> MAMKREQTIENLYQLAQLTQQVQADRIEIVLEERRDEHFPPMSKALMETRSGLTRRKLDEAIAKMEEAGHQFTKNNANHYSISLSEAHMLMDAAGVPKFHERKKNNENKPWIINVQNQKGGTGKSMTAVHLAACLALNLDKRYRICLIDLDPQGSLRLFLNPQISLAEHTNIYSAVDIMLDNVPDGVQVDTEFLRKNVMLPTQYPNLKTISAFPEDAMFNAEAWQYLSQNQSLDIVRLLKEKLIDKIASDFDIIMIDTGPHVDPLVWNAMYASNALLIPCAAKRLDWASTVNFFQHLPTVYEMFPEDWKGLEFVRLMPTMFEDDNKKQVSVLTEMNYLLGDQVMMATIPRSRAFETCADTYSTVFDLTVNDFEGGKKTLATAQDAVQKSALELERVLHSHWSSLNQG

Bacterial cells use several evolutionarily-distinct genome segregation systems, the most common of which is the type I Par system. It consists of an adapter protein, ParB, that binds to the DNA cargo via interaction with the parS DNA sequence; and an ATPase, ParA, that binds nonspecific DNA and mediates cargo transport. Each chromosome encodes its own segregation complex, with Chr1 encoding a chromosomal type Ib system, and Chr2 encoding a plasmid-like type Ia system. In this study, we have reported the structure of the ParA2vc protein, in three states: apo, nucleotide-bound (ADP) and in a filamentous complex with nucleotide and DNA.

The purified protein crystallized readily, and the obtained crystals diffracted to ~2.5 Å. The obtained ParA2vc crystal structure includes one ParA2vc molecule per asymmetric unit. The overall structure of the ParA2vc monomer is similar to that of P7 ParA, with an overall RMSD of 2.2 Å for CA atoms. In particular, the N-terminal HTH domain resembles that of P1 and P7 ParA, confirming that ParA2vc belongs to the type Ia family. No ligand density was observed in the active site, confirming that this structure corresponds to the apo state of the protein. It is worth noting that the nucleotide-binding site is generally poorly resolved, and in particular we were not able to build the P-loop in this structure. One of the symmetry-related pairs is consistent with a biological dimer, and largely resembles the P7 ParA dimer structure. This suggests that we have obtained the structure of the ParA2vc dimer through crystallographic symmetry. Comparing the ParA2vc dimer to that of the P7 ParA structure confirms that they possess a similar architecture, with helix 1 forming a domain-swapped interaction with the adjacent subunit. Overall, this structure confirms the common architecture of ParA proteins, and is consistent with the fact that the V. cholerae chromosome 2 is plasmid-like, as suggested previously, since the ParA2vc structure confirms that it belongs to the type Ia family.>[2x]FQGSESQLSVRVTPANAALKANIEAYVGSLGERDEAALQRFRRNAEAQAEKAAQALGYFQAQIDSEVKDGKPPKLTLKVVPGEPVRLRQVNIQVLGEAASLESFRLPSGKQLKPGAKLNQGVYEDAKRLIQNQASRYGFFQGRFSTQRLSIDPRAGIADIDLVYDSGQRYTFGKVSFDGDSIIEEELLRRMVPFKAGQPYDSELIAELNQNLQSSGYFEGVRVDAAPTQAQADGARQAIPVAVRLEARKPRTMGVGLGFSTDVGARARFNWTRHWVNAEGHSLGFESEISAPRQNVGAWYEIPLDPPLTDKLRFTSGYQFED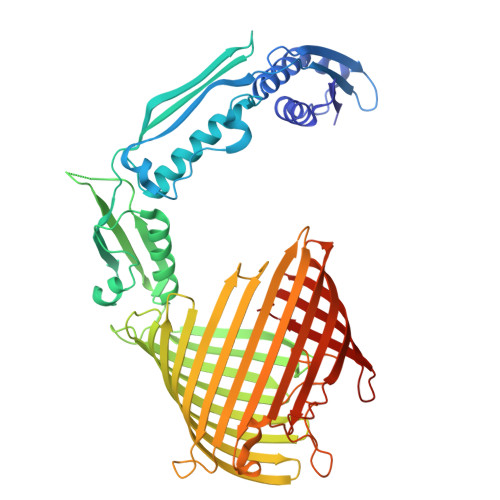LVDTESKLLTLGGEWHSKRPDGWQRVVSLNWMREEYKLGDDSGLSSFLMPGIGYSLLETDNKVDPSHGYRLQFNVKGAKEGLLADADVLHVDAMAKGLTSFAGGHRLLGRLQVGGIATNDYKSIPPSLRFFAGGDQSVRGYDYRTLSPENSDGDKIGGRYMIAGSVEYQYPLAERWRLATFVDQGNAFNSLDFPSIKTGVGFGVRWVSPVGPLRLDLAHALDDDGGFRLHFSMGPEL3-(1H-indol-3-yl)-4-[2-(4-oxopiperidin-1-yl)-5-(trifluoromethyl)pyrimidin-4-yl]-1H-pyrrole-2,5-dione 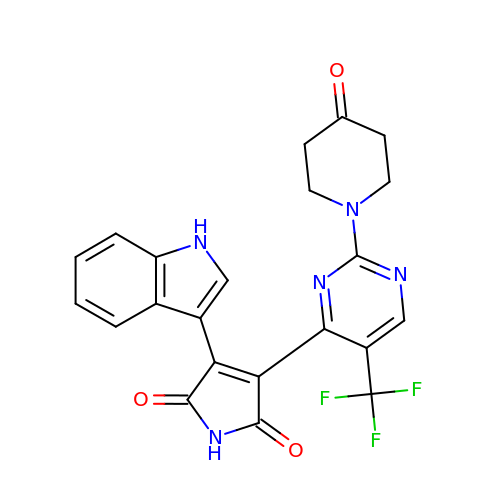| C22 H16 F3 N5 O3 | MYIILBMNTUDZDH-UHFFFAOYSA-N>[2x]SNAELESEALGLQAYKNQMSKQQLLGEIQGFKENYWNMKDLLTLTNRHHLRVFLEYLDNICSAFKDDKTDEKSARAAYDFLNAQINKLFEDNSKNSKPSFESFSEDVQRFLIHIDT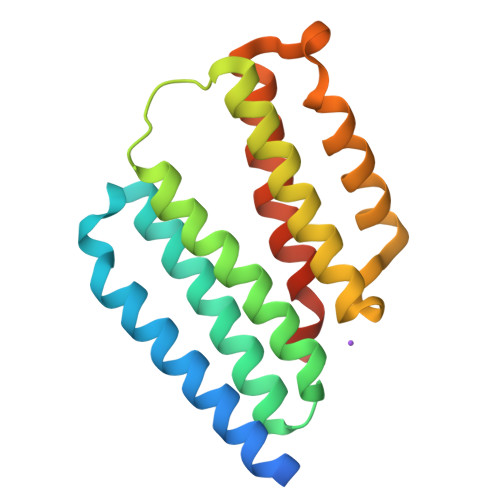YLMKNPSACSNSIASTIQLLKQLDNKKSFNPEQSFKDFCSYKEITIQLLLKPFETPVAEMAS> GAACGGDDKGGAKTAEGNKTGITYPEIKLGETGKDIKTTITFMNNRTDMNLDTYPGKNWKSYIEDFNKMYPNITVKVQTDSNYADSALTRLQANNDSWDIMMIPAVDKSEFSNYFVPYGETSEMEKVIKLADEKAYDGQTYGIANNGVTAGIVYNKKVFEEAGIKELPKTPEEFQADLKLIKEKTKAVPLYT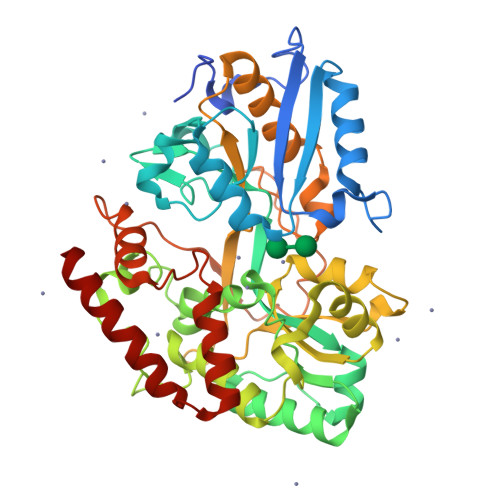NFVEDWAMGAWDQYIAGNATGDPKFMNQVLPTTKEPFKKDASAPDTHPYAVYKTLYDAVANGYTEEDYSTTDWESSKGKMNNGEIATMVLGAWAVPQMKQAGDHPDDIGYMPFPITVDGKQYATIAGDYSYGINKNISKEKQEASMIFVKWMTEDSGFAKNEGGIPIKADDESMPETYETFSDVELITDAPAKEGQEDLLANVNSDSELGINNGNGKKIQDIVVDAANRTRTIDQIMDEWNQKWAKAVEDNE> DLLSCLTFNGVRNHTVFSADSDSDFNRFLHLSIQNPLFQNSLISKPSAIILPGSKEELSNTIRCIRKGSWTIRLRSGGHSYEGLSYTSDTPFILIDLMNLNRVSIDLESETAWVESGSTLGELYYAITESSSKLGFTAGWCPTVGTGGHISGGGFGMMSRKYGLAADNVVDAILIDANGAILDRQAMGEDVFWAIRGGGGGVWGAIYAWKIKLLPVPEKVTVFRVTKNVAIDEATSLLHKWQFVAEELEEDFTLSVLGGADEKQVWLTMLGFHFGLKTVAKSTFDLLFPELGLVEEDYLEMSWGESFAYLAGLETVSQLNN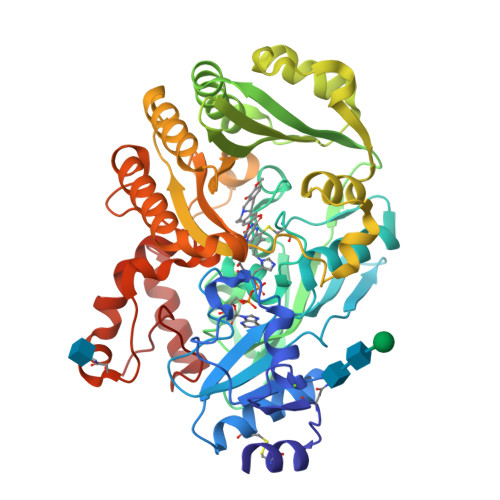RFLKFDERAFKTKVDLTKEPLPSKAFYGLLERLSKEPNGFIALNGFGGQMSKISSDFTPFPHRSGTRLMVEYIVAWNQSEQKKKTEFLDWLEKVYEFMKPFVSKNPRLGYVNHIDLDLGGIDWGNKTVVNNAIEISRSWGESYFLSNYERLIRAKTLIDPNNVFNHPQSIPPMA>[2x]GPPLPEELVLLERTLADGSTEQIIFSSAGDVNVYDLQALCDKV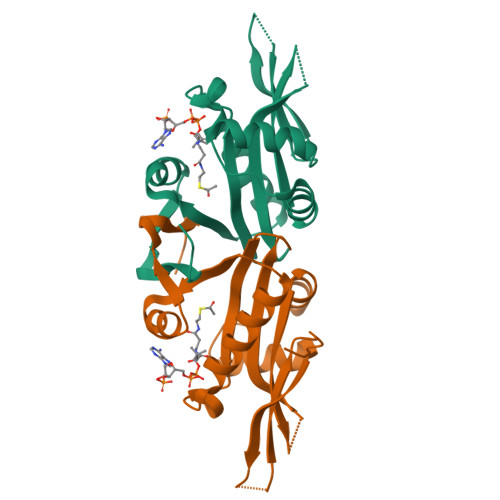GWPRRPLTKIAASLRNSYLVATLHSVTMPSKAEGEERKQLIGMARATSDHAFNATIWDVLVDPSYQGQGLGKALMEKVIRTLLQRDISNITLFADNKVVDFYKNLGFEADPQGIKGMFWYPRF>[4x]MTMDEQQSQAVAPVYVGGFLARYDQSPDEAELLLPRDVVEHWLHAQGQGQPSLSVALPLNINHDDTAVVGHVAAMQSVRDGLFCLGCVTSPRFLEIVRRASEKSELVSRGPVSPLQPDKVVEFLSGSYAGLSLSSRRCDDVEQATSLSGSETTPFKHVALCSVGRRRGTLAVYGRDPEWVTQRFPDLTAADRDGLRAQ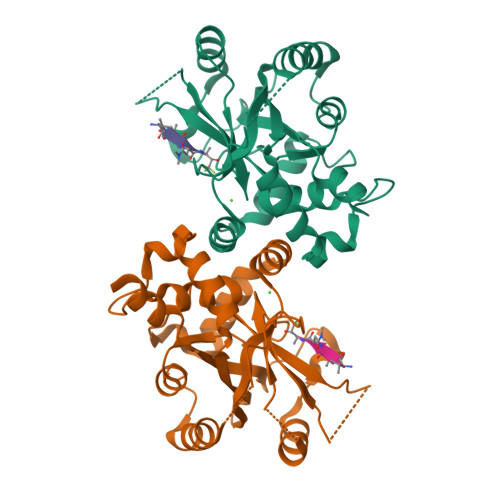WQRCGSTAVDASGDPFRSDSYGLLGNSVDALYIRERLPKLRYDKQLVGVTERESYVKA> G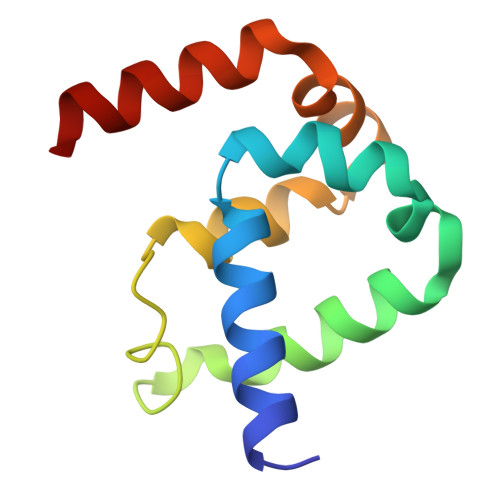NRLRFQLELEFVQCLANPNYLNFLAQRGYFKDKAFVNYLKYLLYWKEPEYAKYLKYPQCLHMLELLQYEHFRKELVNAQCAKFIDEQQILHW> MTMDATALPSELLVTPQPLVGFCGLDTARVSVHKAVWEAFSGSLQRKAADRAAVQYKLLP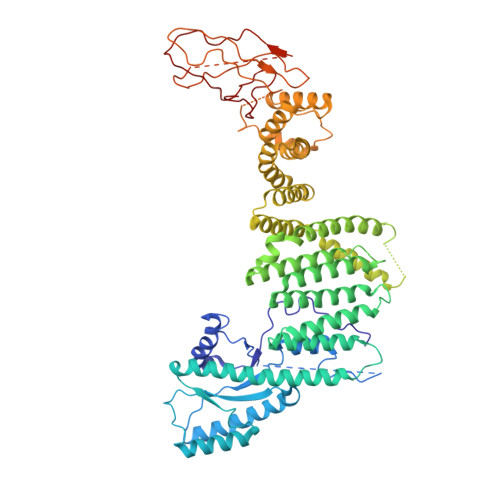PNYEFPVAKPKRASYEWYHPKGILKRNWMLKHLHVLPSVVVLFQDMEWNDLQWTEKQVQCAAIVQALKNTLQERNTRLCLVLLQRAAPLPPGEDLLAAERAASLTNACGITSKMLFILPHTEHLTGYALRLESAFLDMAQSYYALMSKRIRNHRDQLTAAHTSLKIRHQFKLGFVAEMRQDFSTGQKHYFQAYANLDEIRINDGNCLEIKTLAGFLNYKICRLMFKLKTPRDAINQFIIHVEKHKSRVGFKDLAFEHHAWLSTQHSVFAELFCEAIKNGLPALQTQHPGIYYHKAAEFVMKRRDAAMEAYAAMQASSEATPTPIQNPLSLYTEFFGIRAVKTGDLVAEQQANMQLCDQERSYNHSAAIIALLSQAMAQFKIYKCLRFRKKLAIDMAEEYLKSGDHAKALTLYSLMLPDYRQEKWTTIFTDVLLKTLRCALLSGSVADYIACSVEALSLRHQSDQSERILILENLWQVFQGVPPMPKTQLTPEAQALWTSALANVKSPIQIDLDKVNDVVEMCATFERVQLSNDDLLQLQLIVRVLTDIPLRIRSFHVILADAGNPQNSYKLEALKYFCFPTLTQLRGQKQPDDEQLENPSQEPKNFEKNMRLEPGSYYQLFCSTEAQQFHENTQLRIVRLEAHMGTDQVAALLTCSSN> MDVAGLTDCGLIRKSNQDAFYIDEKHQRFFIVADGMGGHAGGEEASRLAVDHIRQYL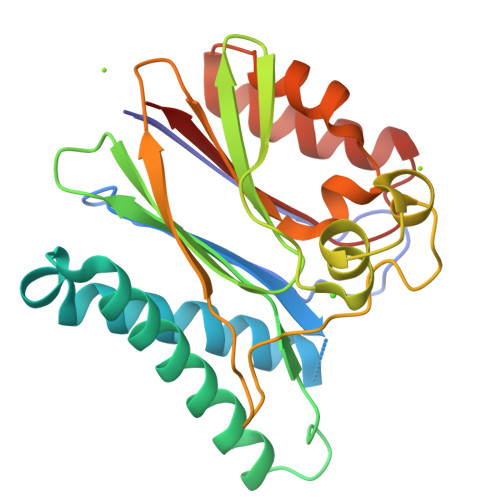ETHLEDLQHDPVTLLRQAFLAANHAIVEQQRQNSARADMGTTAVVILLDEKGDRAWCAHVGDSRIYRWRKDQLQQITSDHTWIAQAVQLGSLTIEQARQHPWRHVLSQCLGREDLSQIDIQPIDLEPGDRLLLCSAGLTEELTDDVISIYLSEPNVQKAAAALVDAAKTHGGRDNVTVVVISV We reported previously that the DNA repair enzyme aprataxin has a DNA 3′ de-capping activity, converting DNAppG to DNA3′p and GMP. Aprataxin catalyzes the conversion of A5′pp5′DNA to AMP and pDNA via a covalent enzyme-(histidinyl)–AMP intermediate. Aprataxin consists of two modules: a proximal HIT domain and a C-terminal zinc-finger. The HIT domain is organized around a central 6-strand antiparallel β-sheet that, along with flanking loops and helices, forms the NMP-binding pocket.

We undertook crystallization trials of aprataxin that had been incubated with two complementary 10-mer DNA oligonucleotides, 5′ HOGAATCATAACOH and 5′ HOGTTATGATTCp, that were designed to form a 10-bp blunt duplex with a single 3′-terminal phosphate group. The goal was to capture a DNA complex with the 3′-PO4 strand poised at the active site, in a reverse orientation of the duplex vis à vis previous aprataxin·DNA complexes wherein the DNA 5′-OH terminus was at the active site. Crystals were obtained in space group P321. The structure of the complex was refined at 2.25 Å resolution to R/Rfree of 18.0/24.0. The asymmetric unit contained one aprataxin protomer and one copy of the HODNAOH strand. A second copy of each was situated at a crystallographic two-fold, so that the two DNA strands formed a 10-nt blunt duplex, albeit with 8/10 base mismatches, the terminal G:C pair being the only one with canonical Watson–Crick configuration. An aprataxin protomer was engaged at each end of the duplex, with the 5′-OH terminus of the ‘substrate strand’ projecting toward the active site. The duplex end is bookmarked by Phe34, which makes a π-stack on the guanine nucleobase of the 5′ G:C base pair. Lys67 and His165 coordinate the terminal phosphodiester of the substrate strand and Lys161 coordinates the second phosphodiester. The structure we did obtain, in a 5′-OH orientation, echoes those reported previously and underscores the theme that fission yeast aprataxin favors crystallization with the enzyme bound to both 5′-OH duplex ends, seemingly independent of a specific duplex length or a requirement for canonical nucleobase pairing.

> SFRDNLKVYIESPESYKNVIYYDDDVVLVRDMFPKSKMHLLLMTRDPHLTHVHPLEIMMKHRSLVEKLVSYVQGDLSGLIFDEARNCLSQQLTNEALCNYIKVGFHAGPSMNNLHLHIMTLDHVSPSLKNSAHYISFTSPFFVKIDTPTSNLPTRGTLTSLFQEDLKCWRCGETFGRHFTKLKAHLQEEYDDWLDKSVSM> AKVVCVLYDDPINGYPTSYARDDLPRIDKYPDGQTLPTPKAIDFTPGALLGSVSGELGLRKYLESQGHELVVTSSKDG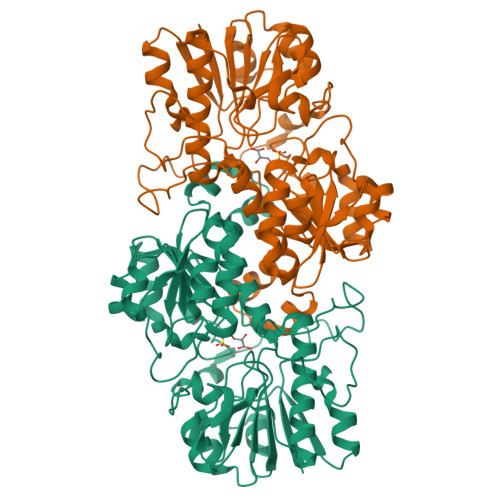PDSELEKHLHDAEVIISQPFWPAYLTAERIAKAPKLKLALTAGIGSDHVDLQAAIDNNITVAEVTYCNSNSVAEHVVMMVLGLVRNYIPSHDWARNGGWNIADCVARSYDVEGMHVGTVAAGRIGLRVLRLLAPFDMHLHYTDRHRLPEAVEKELNLTWHATREDMYGACDVVTLNCPLHPETEHMINDETLKLFKRGAYLVNTARGKLCDRDAIVRALESGRLAGYAGDVWFPQPAPNDHPWRTMPHNGMTPHISGTSLSAQTRYAAGTREILECYFEGRPIRDEYLIVQGGGLAGVGAHSYSKGNATGGSEEAAKYEKLDA>[2x]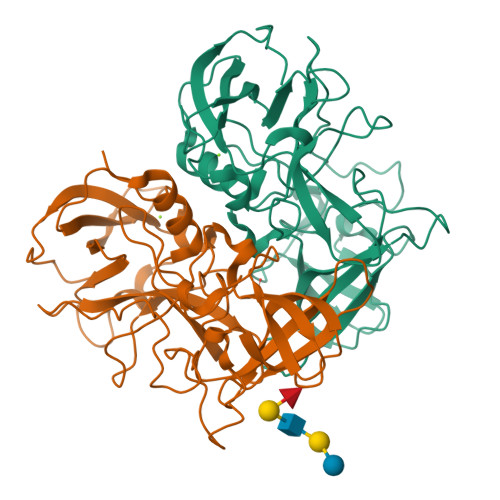EQKTRPFTLPNLPLSSLSNSRAPLPISSMGISPDNVQSVQFQNGRCTLDGRLVGTTPVSLSHVAKIRGTSNGTVINLTELDGTPFHPFEGPAPIGFPDLGGCDWHINMTQFGHSSQTQYDVDTTPDTFVPHLGSIQANGIGSGNYVGVLSWISPPSHPSGSQVDLWKIPNYGSSITEATHLAPSVYPPGFGEVLVFFMSKMPGPGAYNLPCLLPQEYISHLASEQAPTVGEAALLHYVDPDTGRNLGEFKAYPDGFLTCVPNGASSGPQQLPINGVFVFVSWVSRFYQLKPVGTA>[2x]AQTVPYGIPLIKADKVQAQGFKGANVKVAVLDTGIQASHPDLNVVGGASFVAGEAYNTDGNGHGTHVAGTVAALDNTTGVLGVAPSVSLYAVKVLNSSGSGSYSGIV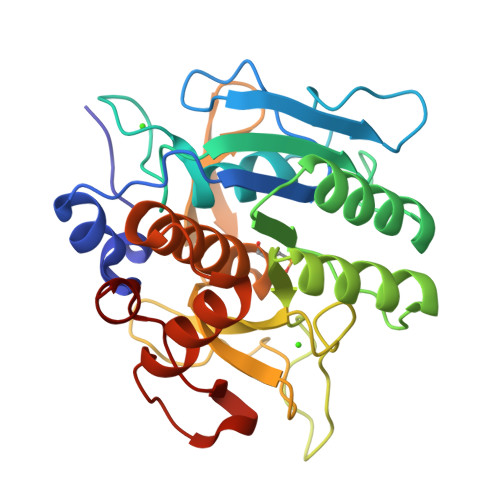SGIEWATTNGMDVINMSLGGASGSTAMKQAVDNAYARGVVVVAAAGNSGNSGSTNTIGYPAKYDSVIAVGAVDSNSNRASFSSVGAELEVMAPGAGVYSTYPTNTYATLNGTUMASPHVAGAAALILSKHPNLSASQVRNRLSSTATYLGSSFYYGKGLINVEAAAQ>GMSTDTCIKRPTRSELVDRFQKKIRAGEPIIGGGAGTGLSAKSEEAGDIDLIVIYNSGRYRMAGRGSLAGLLAYGNANQIVVDMAREVLPVVRHTPVLAGVNGTDPFMVMSTFLRELKEIGFAGVQNFPTVGLIDGLFRQNLEETGMSYAQEVEMIAE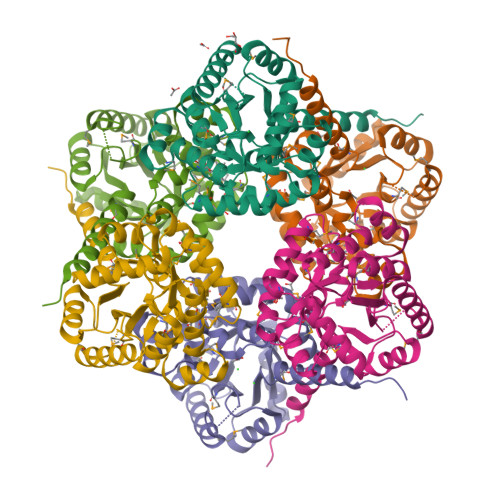AHKLDLLTTPYVFSPEDAVAMAKAGADILVCHMGLTTGGAIGARSGKSMDDCVSLINECIEAARTIRDDIIILSHGGPIANPEDARFILDSCQGCHGFYGASSMERLPAEEAIRSQTLAFKAIRRQPA[6x]>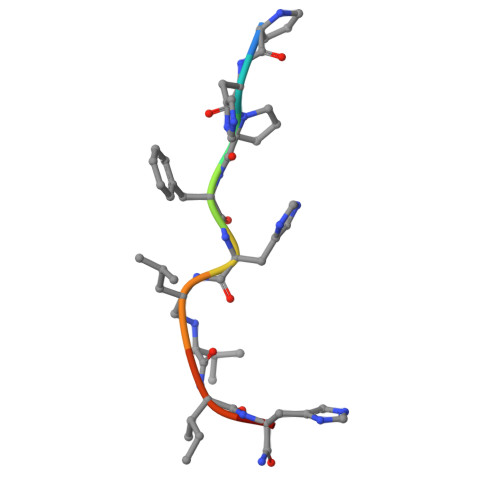 PHPFHXIHK>[2x]VGPIQSIKVDPMKSGGLGVVYRSPDKGRVSLYLYNDGEDILLVVDARFDWRGEQNVLVLNSKFAGGEWGPEVRPEGFPFPCCGYVTTITVRVEI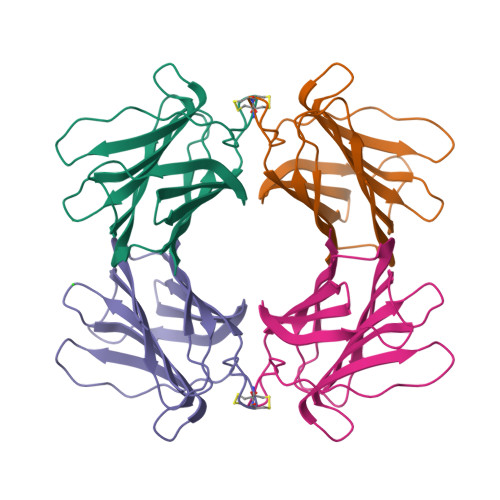GADGFTLSANGIEIVKYPYRDGLPPPVTKFQYVFQDQGASETAQLESLSAYY>MGAAPDSHQLAKALAEAADVGAQMIKLVGLRELSEAERQLRSLVVALMQEVFTEFFPGCVVHPFGSSINSFDVHGCDLDLFLDLGDLEEPQPVPKLPPASPLLEDREEGDLGKASELAETPKEEKAEGAAMLELVGSILRGCVPGVYRVQTVPSARRPVVKFAHRPSGLHGDVSLSNRLALHNSRFLSLASELDGRVRPLVYTLRAWAQGRGLSGSGPLLSNYALTLLVIYFLQTRDPPVLPTVSQLTQKAGEGEQVEVDGWDCSFPRDASRLEPSINVEPLSSLLAQFFSAVSSWDLRGSLLSLREGQALPVAGGLPSNLWEGLRLGPLNLQDPFDLSHNVAANVTSRVAGRLQNCCRAAANYARSLQYQRRSSRGRDWGLLPLLQPSSPSSLLSATPIPLPLAPFT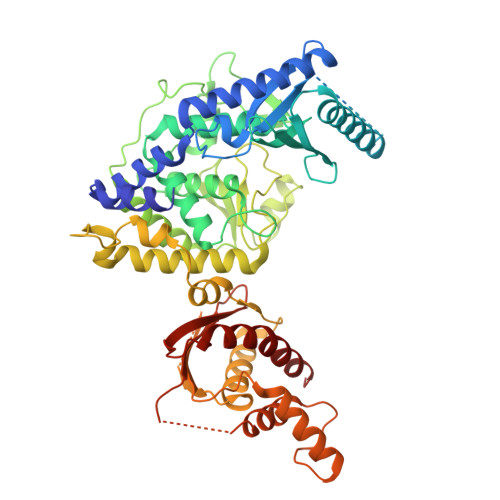QLTAALVQVFREALGCHIEQATKRTRSEGGGTGQGEAGKGASLPSSASWRCALWHRVWQGRRRARRRLQQQTKEGAGGGAGTRAGWLATEAQVTQELKGLSGGEERPETEPLLSFVASVSPADRMLTVTPLQDPQGLFPDLHHFLQVFLPQAIRHLKLEHHHHHH[2x]> AGGCCTAGCCTGTACGGA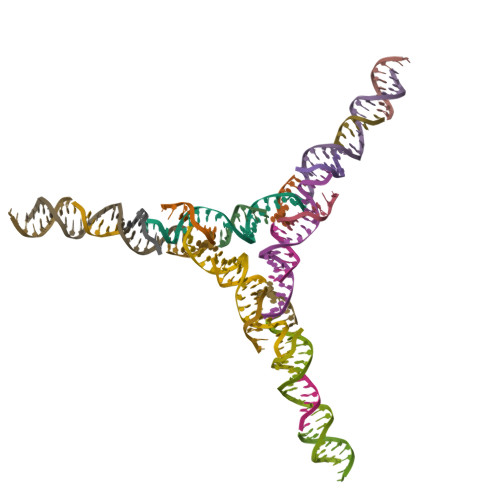CATCAG;>[2x]CCGTACA;> GGCTAGGC;>TCCTGATGT[2x];> AGGCCTACCCTGTACGGACATCAG;> GGCTAAGC> MSLDGTELRLKGEKLRYVSRGGLKLEKALKEFHLEINGKTCLDIGSSTGGFTDVMLQNGAKLVYALDVGTNQLAWKIRSDERVVVMEQFNFRNAVLADFEQGRPSFTSIDVSFISLDLILPPLYEILEKNGEVAALIKPQFEAGREQVGKNGIIRDPKVHQMTIEKVLKTATQLGF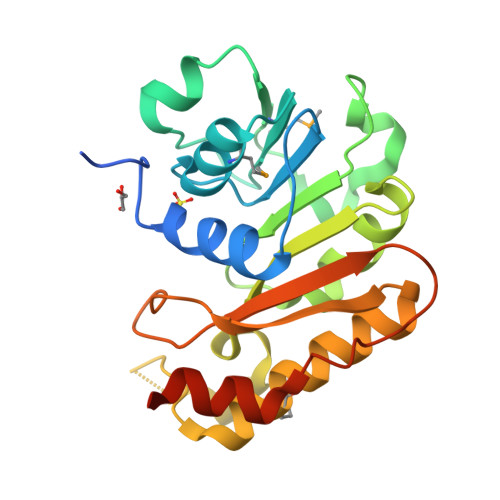SVKGLTFSPIKGGAGNVEFLVHLLKDGKAEIAQQVNIESVLQKESEELEGHHHHHH> MKHHHHHHHHGGLVPAGSHGGMQRPIVYVGMSADLIHPGHINILSRAAELGDITIGLLTDAAIASYKRLPHMTYEQRKAVVENLKGVASVVPQRTLDYAENLRTVRPDFVV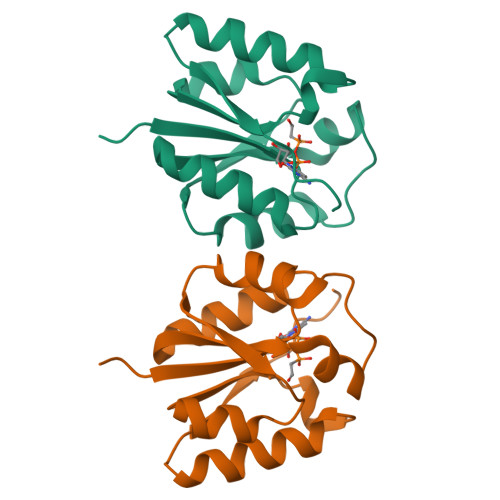HGDDWQTGVQRHTRERVIEVLSEWGGKLVEIPYTPGISSTRLHSSVKEV> SNAATETAILEGWPTLQEVLEDSFMKRLLRCYLSDERSEENLDFLESVGLYESQFDKLTPKVRLEALNFIKDQFLDRNSERQVNLSYQIQQSILKKLSEVTSNAPKDVFNEAKKATEYLLYTEQYTYFINKLNANTIGTGKKDVYSLYLNQFPKTNPQPLYKPTLNKIIEIEKKSWNEDEVKRNTESIKSLVESLIQDECNYVGVLTSLSEFSEIMTKKQILGPDVLKELFDHIPVLIQHHQKFISSLQEAKADEKVGEKLNSGLHFLVLYRYYLRHVPKNIAKLCSIGMTDEIEVGRELYPLPVIEEFDKQQKMTKKMSVLQMLVYPYFRVR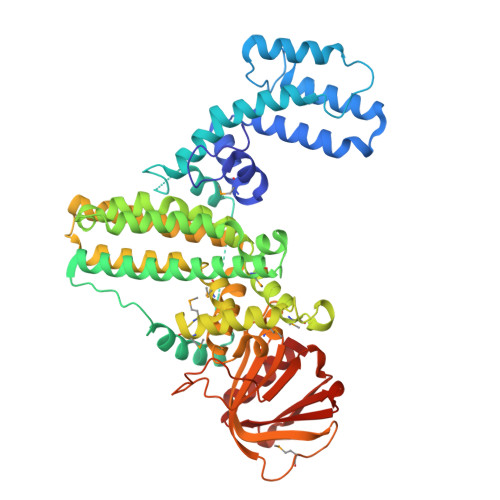TYQAYVDDFIKITKKDSQEVKELEVVHSQLAIFQELINTYSDINKIERISDALKLLFPFSFTSIMPLFEGKNGICGIASLDRFDKTDINQLSMSLNSRKKLTLIILYRGVVVTDVPVIRKKGNVSNSIDKSFYSFTLIGDIRDFGTEDSTETIYIDVPEIKKRIWFGCESTEEFKSCVEALRTIL>[2x]TLGNTTSSVILTNYMDTQYYGEIGIGTPPQTFKVVFDTGSSNVWVPSSKCSRLYTACVYHKLFDASDSSSYKHNGTELTLRYSTGTVSGFLSQDIITVGGITVT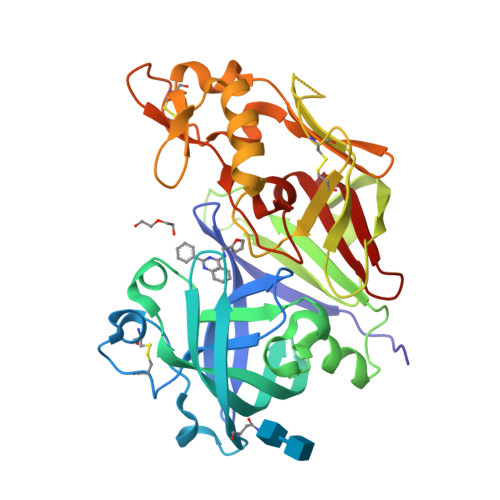QMFGEVTEMPALPFMLAEFDGVVGMGFIEQAIGRVTPIFDNIISQGVLKEDVFSFYYNRDSENSQSLGGQIVLGGSDPQHYEGNFHYINLIKTGVWQIQMKGVSVGSSTLLCEDGCLALVDTGASYISGSTSSIEKLMEALGAKKRLFDYVVKCNEGPTLPDISFHLGGKEYTLTSADYVFQESYSSKKLCTLAIHAMDIPPPTGPTWALGATFIRKFYTEFDRRNNRIGFALAR>[3x]LSSPADSYNEGVKLQPQEISPPPTANLDRSNDKVYENVTGLVKAVIEMSSK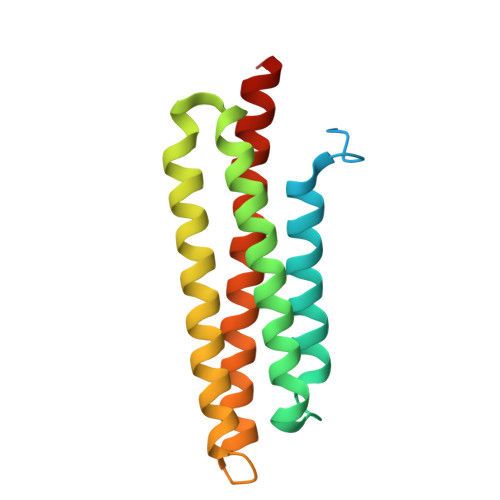IQPAPPEEYVPMVKEVGLALRTLLATVDETIPLLPASTHREIEMAQKLLNSDLGELINKMKLAQQYVMTSLQQEYKKQMLTAAHALAVDAKNLLDVIDQARLKMLGQTRPH[(3R)-3-aminopiperidin-1-yl][2-(1-ethyl-1H-pyrrolo[2,3-b]pyridin-2-yl)-7-methoxy-1-methyl-1H-benzimidazol-5-yl]methanone | C24 H28 N6 O2 | 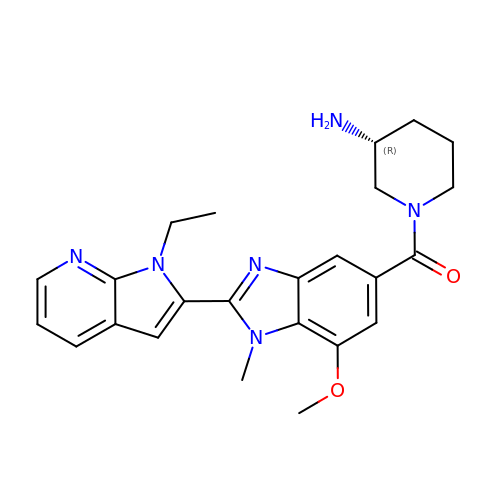JCCVZBCVMBEDEN-QGZVFWFLSA-N>HTRMFSVWVNGVDQGDGQNVYIRTPPNTDPIKDLASPALACNVKGGEPVPQFVSASAGDKLTFEWYRVKRGDDIIDPSHSGPITTWIAAFTSPTMDGTGPVWSKIHEEGYDASTKSWAVDKLIANKGMWDFTL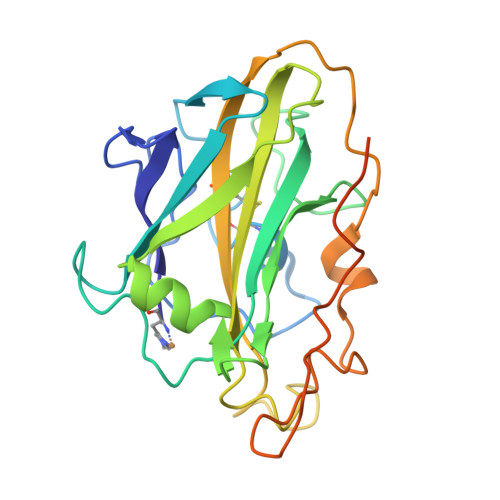PSQLKPGKYMLRQEIVAHHESDATFDKNPKRGAQFYPSCVQVDVKGVGGDAVPDQAFDFNKGYKYSDPGIAFDMYTDFDSYPIPGPPVWDAQDEGCCFIDGVDTTSVKEVVKQIICVLK[6x]> MIRFKKTKLIASIAMALCLFSQPVISFSKDITDKNQSIDSGISSLSYNRNEVLASNGDKIESFVPKEGKKAGNKFIVVERQKRSLTTSPVDISIIDSVNDRTYPGALQLADKALVENRPTILMVKRKPININIDLPGLKGENSIKVDDPTYGKVSGAIDELVSKWNEKYSSTHTLPARTQYSESMVYSKSQISSALNVNAKVLENSLGVDFNAVANNEKKVMILAYKQIFYTVSADLPKNPSDLFDDSVTFNDLKQKGVSNEAPPLMVSNVAYGRTIYVKLETTSSSKDVQAAFKALIKNTDIKNSQQYKDIYENSSFTAVVLGGDAQEHNKVVTKDFDEIRKVIKDNATFSTKNPAYPISYTSVFLKDNSVAAVHNKTDYIETTSTEYSKGKINLDHSGAYVAQFEVAWDEVSYD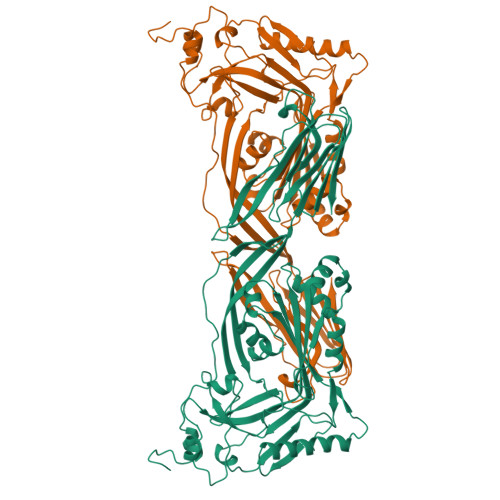KEGNEVLTHKTWDGNYQDKTAHYSTVIPLEANARNIRIKARECTGLAWEWWRDVISEYDVPLTNNINVSIWGTTLYPGSSITYN>[3x]MKIMMSRRELKEEYKQLEGHPEVKSRIKARMRELAKSRMMAEVPKATVVITN;>PTHIAIALKYNPEKDKAPVVVAKGKGTIAQKIVEIAENY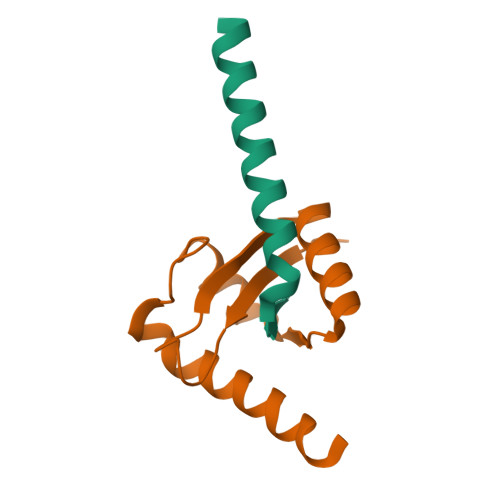SIPVVRKPELARALYPAVEVGKEISPKFYKAVAEIIAYVMFKKKKVYA[3x]>[2x]FSCNVDGGSSIGAGTTSVYVNLDPVIQPGQNLVVDLSQHI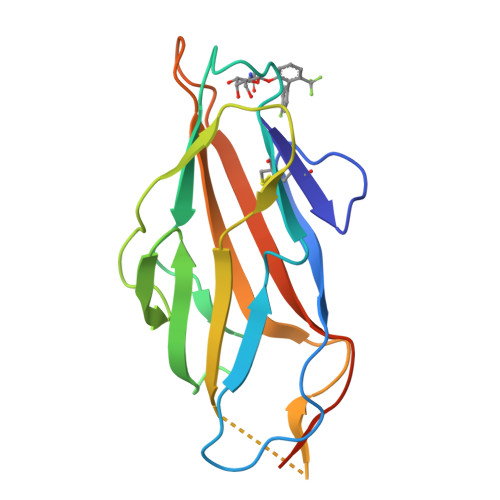SCWNDYGGWYDTDHINLVQGSAFAGSLQSYKGSLYWNNVTYPFPLTTNTNVLDIGDKTPMPLPLKLYITPVGAAGGVVIKAGEVIARIHMYKIATLGSGNPRNFTWNIISNNSVVMPTGGHHHHHH> SNANDAAEVALYERLLQLRVLPGASDVHDVRFVFGDDSRCWIEVAMH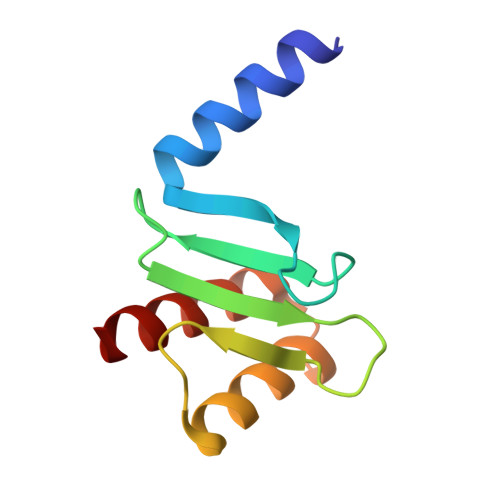GDHVIGNSHPALDPKSRATLEHVLTVQGDLAAFLVVARDMLLASL> MTWSYPVDPYWMVALKALLVVVGLLTAFAFMTLIERRLLARFQVRMGPNRVGPFGLLQPLADAIKSIFKEDIVVAQADRFLFVLAPLISVVFALLAFGLIPFGPPGSFFGYQPWVINLDLGILYLFAVSELAVYGIFLSGWASGSKYSLLGSLRSSASLISYE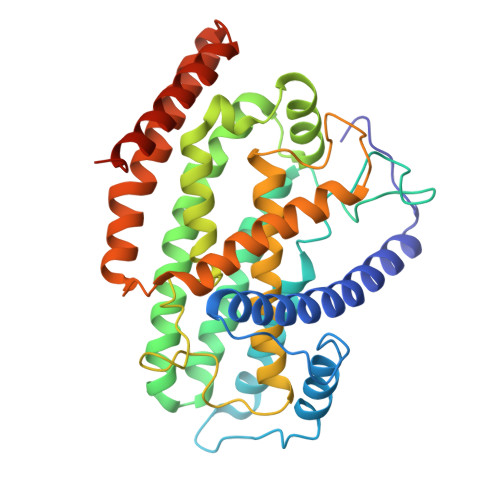LGLGLALLAPVLLVGSLNLNDIVNWQKEHGWLFLYAFPAFLVYLIASMAEAARTPFDLPEAEQELVGGYHTEYSSIKWALFQMAEYIHFITASALIPTLFLGGWTMPVLEVPYLWMFLKIAFFLFFFIWIRATWFRLRYDQLLRFGWGFLFPLALLWFLVTALVVALDLPRTYLLYLSALSFLVLLGAVLYTPKPARKGGGA>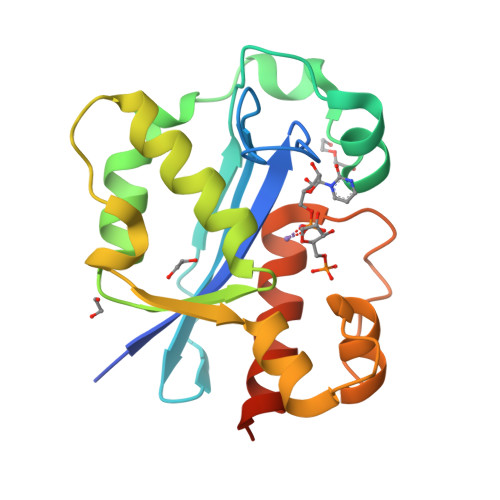 SIEFSTAITRQIVLDTETTGMNQIGAHYEGHKIIEIGAVEVVNRRLTGNNFHVYLKPDRLVDPEAFGVHGIADEFLLDKPTFAEVADEFMDYIRGAELVIHNAAFDIGFMDYEFSLLKRDIPKTNTFCKVTDSLAVARKMFPGKRNSLDALCARYEIDNSKRTLHGALLDAQILAEVYLAMTGGQTSMATRESG>AGNKSVVYHGTRDLRVETVPYPKLEHNNRKLEHAVILKVVSTNICGSDQHIYRGRFIVPKGHVLGHEITGEVVEKGSDVELMDIGDLVSVPFNVACGRCRNCKEARSDVCENNLVNPDADLGAFGFDLKGWSGGQAEYVLVPYADYMLLKFGDKEQAMEKIKDLTLISDILPTGFHGCVSAGVKPGSHVYIAGAGPVGRCAAAGARLLGAACVIVGDQNPERLKLLSDAGFETIDLRNSAPLRDQIDQILGKPEVDCGVDAVGFEAHGLGDEANT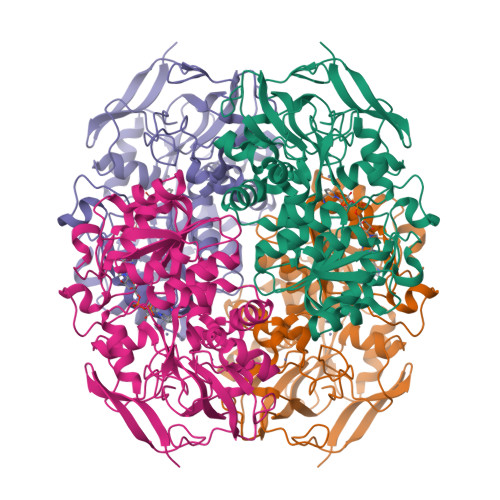ETPNGALNSLFDVVRAGGAIGIPGIYVGSDPDPVNKDAGSGRLHLDFGKMWTKSIRIMTGMAPVTNYNRHLTEAILWDQMPYLSKVMNIEVITLDQAPDGYAKFDKGSPAKFVIDPHGMLKNK[2x]> MEILRYLMDPDTFTSNFNNDPLVLRRRQTYLCYEVERLDNGTSVKMDQHMGFLCNESGRHAQLRFLDLVPSLQLDPAQIYRVTWFISWSPCFSWGCAGEVRAFLQENTHVRLRIKAARIYDDQGRCQEALQMLRDAGAQVSIMTYDEFEYCWDTFVYRQGCPF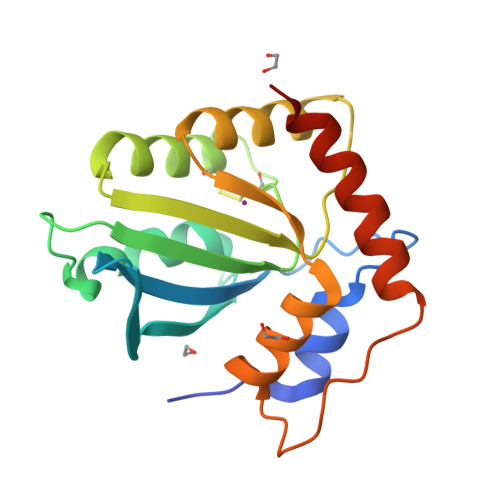QPWDGLEEHSQALSGRLRAILQLEHHHHHH>[2x]MSSHHHHHHSSGLVPRGSHMTDQ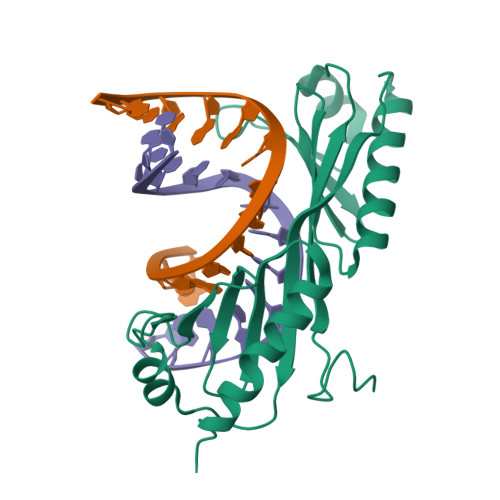GLEGSNPVDLSKHPSGIVPTLQNIVSTVNLDCKLDLKAIALQARNAEYNPKRFAAVIMRIREPKTTALIFASGKMVCTGAKSEDFSKMAARKYARIVQKLGFPAKFKDFKIQNIVGSCDVKFPIRLEGLAYSHAAFSSYEPELFPGLIYRMKVPKIVLLIFVSGKIVITGAKMRDETYKAFENIYPVLSEFRKIQQ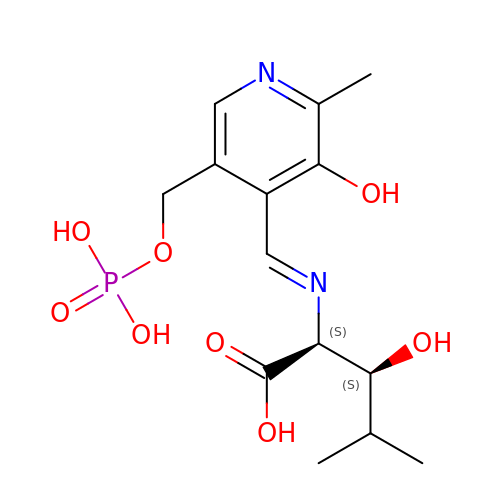(2S,3S)-3-hydroxy-2-[(E)-({3-hydroxy-2-methyl-5-[(phosphonooxy)methyl]pyridin-4-yl}methylidene)amino]-4-methylpentanoic acid (non-preferred name) | C14 H21 N2 O8 P | VDGFQULJGQPRGZ-BGTSGQOBSA-N>ADLANGAKVFSGNCAACHMGGGNVVMANKTLKKEALEQFGMYSEDAIIYQVQHGK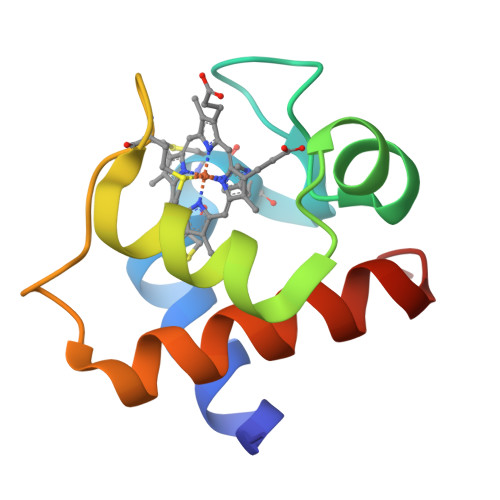NAMPAFAGRLTDEQIQDVAAYVLDQAAKGWAG[6x]Protein A075L is a β‐xylosyltransferase that participates in producing the core of the N‐glycans found in VP54, the major viral capsid protein of Paramecium bursaria chlorella virus‐1 (PBCV‐1). The protein structure shows a typical GT‐B folding, with two Rossmann‐like fold domains, in which the acceptor substrate binds to the N‐terminal region, and the nucleotide‐sugar donor binds to the C‐terminal region. We propose that the catalytic mechanism follows a direct displacement SN2‐like reaction, where Asp73 serves as a catalytic base that deprotonates the incoming nucleophile of the acceptor, facilitating direct displacement of the UDP with the inversion of the anomeric configuration of the acceptor without metal ion dependence, while the interactions with side chains of Arg158 and Arg208 stabilize the developing negative charge. In this context, we herein present the structural and biochemical characterization of A075L, a soluble chlorovirus xylosyltransferase easily produced in E. coli and amenable to large‐scale purification.

To address the enzymatic mechanism, we solved the 3D structure of A075L in its apo form as well as in its complexes with the donor 1 and the trisaccharide 6 acceptor. The structural analysis of these structures revealed that A075L adopts a GT‐B fold, comprising two Rossman‐like domains. The active site is located between these two domains; the N‐terminal domain is responsible for the glycan acceptor coordination, whereas the C‐terminal domain binds the UDP‐sugar donor. In contrast to its earlier classification as an exostosin (PF03016) within the GT47 family (Speciale et al. 2019), we show that the region spanning from V66 to K222 does not constitute an independent domain. Instead, this region comprises the β‐sheet of the N‐terminal Rossmann domain and several helices at the C‐terminal domain, as shown in Figure S3e. Despite several attempts to co‐crystalize A075L with both the acceptor and the donor molecules simultaneously, none were successful. The reaction occurred so rapidly that we consistently obtained the apo form without the bound product or intermediate, even when using the A075LD73N mutant. Despite extensive screening, only crystals with an empty active site or no crystals at all were obtained.

>[8x]GPLGSMKLAELTLESDDFITSDKLFNFCKSTIFGAKYVKTDFIKFRQYQYIVSNCGWRDDTDVVFLENTPVLVTGHSDYDISEREIDIIRLPNIRAWFCQNRNIPHPKVISFPLGITNKDEPNSEIHRIIGNTDRILEVSKTPKEIKNLVYMNITVKNFPEERQRIVDLYSDKSWVTIGKGEVSEEGHRKFLEDMYAHKFCFAPRGNGIDTHRLWESLYLRTIPIVKKHIAMEQFTDLPILFVNDWENITEEYLNEQYDIIMAKDWNLDKLKIDYWYQKILEYSQ>[2x]SNADLSLEQRVGQLFMVGTDAATAEQVTLDAITASHVGNVFLAGRSN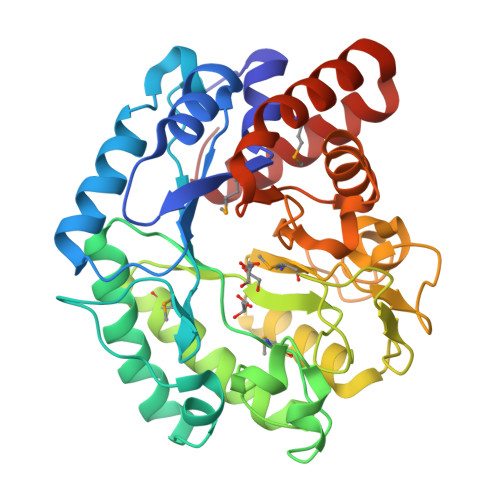AGVDATAAVVEQLTAAVTDEATGGVPLLVATDQEGGNVQVLRGPGFSDIPTALDQGALDPATLQADATTWGAELAASGINLNLAPVMDVVASPEAAAANPPIGYFHREFGYDAETVASHANAFSAGMRASGVETVIKHFPGLGRVTENTDTTAGVVDDVTTADDASVQAFAAGIDAGAAFVMTSTAVYSQIDPDAPAAFSREIVSDLLRGQLGFDGVVVTDDVSAAEQVQAWSPADRAILAIEAGTDIVLVSADPSIAAEMVAAVVAKAQADPDFAAIVDDAARRVLAAKGVA>[6x]MRGSHHHHHHGSMDKNIIIGAMTALITPFKNGKVDEQSYARLIKRQIENGIDAVVPVGTTGESATLTNEEH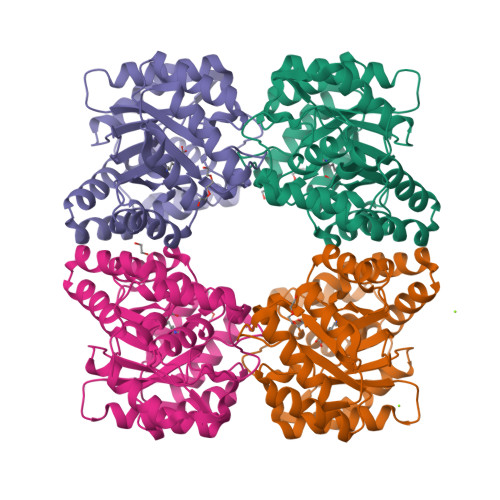RTCIEIAVETCKGTKVKVLAGAGSNATHEAVGLAKFAKEHGADGILSVAPYYNKPTQQGLYEHYKAIAQSVDIPVLLYNVPGRTGCEISTDTIIKLFRDCENIYGVKEASGNIDKCVDLLAHEPRMMLISGEDAINYPILSNGGKGVISVTSNLLPDMISALTHFALDENYKEAKKINDELYNINKILFCESNPIPIKTAMYLAGLIESLEFRLPLCSPSKENFAKIEEVMKKYKIKGF> VFPSSVYVPDEWEVSREKITLLRELGQGSFGMVYEGNARDIIKGEAETRVAVKTVNESASLRERIEFLNEASVMKGFTCHHVVRLLGVVSKGQPTLVVMELMA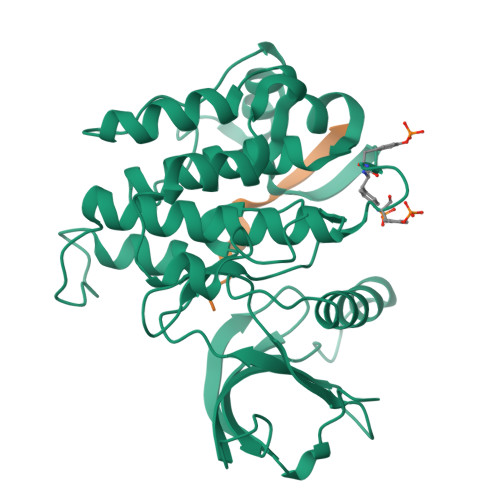HGDLKSYLRSLRPEAENNPGRPPPTLQEMIQMAAEIADGMAYLNAKKFVHRDLAARNCMVAHDFTVKIGDFGMTRDIYETDYYRKGGKGLLPVRWMAPESLKDGVFTTSSDMWSFGVVLWEITSLAEQPYQGLSNEQVLKFVMDGGYLDQPDNCPERVTDLMRMCWQFNPNMRPTFLEIVNLLKDDLHPSFPEVSFFHSEENK;> AYNPYPEDYGDIEIG>[4x]RDMPLDSDVFRVPPGYNAPQQVHITQGDLVGRAMIISWVTMDEPGSSAVRYWSEKNGRKRIAKGKMSTYRFFNYSSGFIHHTTIRKLKYNTKYYYEVGLRNTTRRFSFITPPQTGLDVPYTFGLIGDLGQSFDSNTTLSHYELSPKKGQTVLFVGDLSYADRYPNHDNVRWDTWGRFTERSVAYQPWIWTAGNHEIEFAPEINETEPFKPFSYRYHVPYEASQSTSPFWYSIKRASAHIIVLSSYSAYGRGTPQYTWLKKELRKVKRSETPWLIVLMHSPLYNSYNHHFMEGEAMRTKFEAWFVKYKVDVVFAGHVHAYERSERVSNIAYKITNGLCTPVKDQSAPVYITIGDAGNYGVIDSNMIQPQPEYSAFREASFGHGMFDIKNRTHAHFSWNRNQDGVAVEADSVWFFNRHWYPVDDST

Purple acid phosphatases belong to the family of binuclear metallohydrolases and are involved in a multitude of biological functions, ranging from bacterial killing and bone metabolism in animals to phosphate uptake in plants. Plant PAPs are 110 kDa homodimers, containing Fe(III)-Zn(II) or Fe(III)-Mn(II) centers, and a recombinant isoform from sweet potato has been shown to contain a di-iron center. The characteristic purple color is due to a charge transfer transition between a tyrosine side-chain and the Fe(III). In this study the structures of the rkbPAP-sulfate and rkbPAP-fluoride complexes were determined, providing insight into what we propose are two crucial steps in its catalytic mechanism, (i) the pre-catalytic stage, and (ii) the chemical step.

rkbPAP incubated with fluoride crystallized in a different space group and with different unit cell parameters compared to the sulfate complex. Two dimers in the asymmetric unit are observed yielding four copies of the active site. In these structures the metal ions are on average 3.5 Å apart, a distance significantly larger than that observed in any of the other rkbPAP structures. A small sphere of electron density is observed between the two metal ions, in a position similar, but not identical, to that of the μ-hydroxo in the rkbPAP-sulfate complex. The center of the bridging electron density in the rkbPAP-F structure is 2.5 Å and 2.1 Å from Fe(III) and Zn(II), respectively. Thus, the bridging ligand is shifted 0.2 Å closer to the Zn(II) and 0.4 Å further away from the Fe(III); its distance to the carbonyl oxygen of His323 is 3.6 Å, compared to 3.1 Å observed in the rkbPAP-SO4 structure. These differences indicate that fluoride rather than μ-hydroxide acts as the bridging ligand, as anticipated from kinetic and spectroscopic data collected for PAPs from pig, human and red kidney bean, and other binuclear metallohydrolases. Additional electron densities in the second coordination sphere, close to the fluoride, are tentatively assigned to a sodium ion and a sulfate ion (see Methods section). The sodium ion may offset the charge of the metal bridging fluoride group, and possibly prevents cations (i.e. sulfate, acetate) from binding to the second coordination sphere. However, for the M1 site in the fluoride bound structure the metal ion is shifted by up to 0.4 Å when compared to rkbPAP-SO4 and rkbPAP-PO4 which then results in compensatory rotations of the side chains of Tyr167 and His325. Here, the comparison between the sulfate- and fluoride-bound rkbPAP structures corroborates this mechanism for the activation of the bridging nucleophile.N-[5-(ETHYLSULFONYL)-2-METHOXYPHENYL]-5-[3-(2-PYRIDINYL)PHENYL]-1,3-OXAZOL-2-AMINE 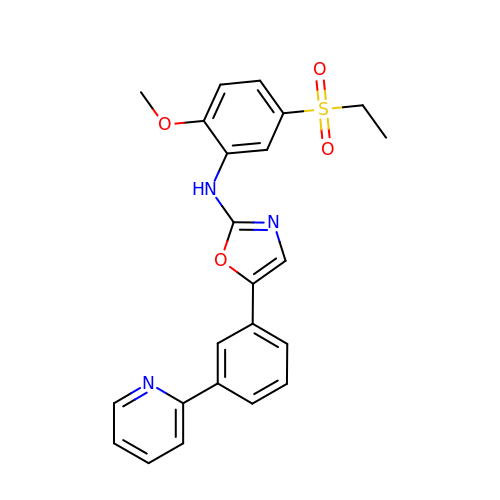| C23 H21 N3 O4 S | HTIZPBXCJPQDEM-UHFFFAOYSA-N> MCTKESEKLNKNADYYIGLDMGTSSAGWAVSDSEYNLIRRKGKDLWGVRQFEEAKTAAERRGFRVARRRKQRQQVRNRLLSEEFQNEITKIDSGFLKRMEDSRFVISDKRVPEKYTLFNDSGYTDVEYYNQYPTIYHLRKALIESNERFDIRLVFLGIHSLFQHPGHFLDKGDVDTDNTGPEELIQFLEDCMNEIQISIPLVSNQKVLTDILTDSRITRRDKEQQILEILQPNKESKKAVSQFVKVLTGQKAKLGDLIMMEDKDTEEYKYSFSFREKTLEEILPDIEGVIDGLALEYIESIYSLYSWSLLNSYMKDTLTGHYYSYLAEARVAAYDKHHSDLVKLKTLFREYIPEEYDNFFRKMEKANYSHYIGSTEYDGEKRCRTAKAKQEDFYKSINKMLEKIPECSEKTEIQKEIIEGTFLLKQTGPQNGFVPNQLQLKELRKILQNASKHYPFLTEKDERDMTAIDRIEALFSFRIPYYIGPLKNTDNQGHGWAVRRDGHEQIPVRPWNFEEIIDESASAD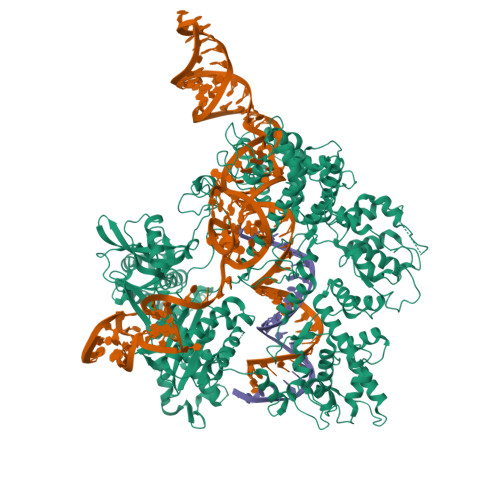LFIKNLVNSCTYLRTEKVLPKSSLLYQEFEVLNELNNLRINGMYPDEIQPGLKRMIFEQCFYSGKKVTGKKLQLFLRSVLTNSSTEEFVLTGIDKDFKSSLSSYKKFCELFGVKTLNDTQKVMAEQIIEWSTVYGDSRKFLKRKLEDNYPELTDQQIRRIAGFKFSEWGNLSRAFLEMEGYKDEAGNPVTIIRALRDTQKNLMQLLSNDSAFAKKLQELNDYVTRDIWSIEPDDLDGMYLSAPVRRMIWQTFLILREVVDTIGYSPKKIFMEMARGEQEKKRTASRKKQLIDLYKEAGMKNDELFGDLESLEEAQLRSKKLYLYFRQMGRDIYSGKLIDFMDVLHGNRYDIDAIHPQSKKKDDSLENNLVLTSKDFNNHIKQDVYPIPEQIQSRQKGFWAMLLKQGFMSQEKYNRLMRTTPFTDEELAEFVNRQLVETRQGTKAIISLINQCFPDSEVVYVKAGNTSDFRQRFDIPKSRDLNNYHHAVDAYLNIVVGNVYDTKFTKNPINFIKKMRKSGNLHSYSLRRMYDFNVQRGDQTAWVAENDTTLKTVKKTAFKTSPMVTKRTYERKGGLADSVLIAAKKAKPGVHLPVKTSDSRFANQVSTYGGYDNVKGSHFFLVEHQQKKKTIRSIENVPIHLKEKLKTKEELEHYCAQVLGMVQPDVRLTRIPMYSLLLIDGYYYYLTGRTGGNLSLSNAVELCLPAKEQAHIRMISKIAGGRSTDALSAEAKDDFRKKNLRLYDELAEKHRSTIFSKRKNPIGPKLLKYREAFVKQTIENQCKVILQILKLTSTNCKTSADLKLIGGSGQEGVMSISKLLRAEKYAEFYLICQSPSGIYETRKNLLTI>GSPGIPGNEKLKEKENNDSSDKATVIPNFNTTMQGSLLGDDSRDYYSFEVKEEGEVNIELDKKDEFGVT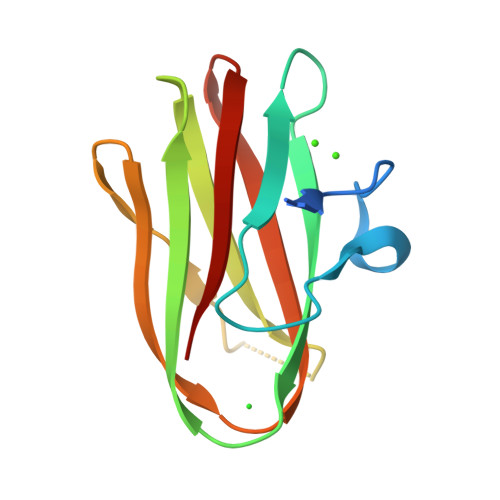WTLHPESNINDRITYGQVDGNKVSNKVKLRPGKYYLLVYKYSGSGNYELRVNK[2x]>QTDMSRKAFVFPKESDTSYVSLKAPLTKPLKAFTVCLHFYTELSSTRGYSIFSYATKRQDNEILIFWSKDIGYSFTVGGSEILFEVPEVTVAPVHICTSWESASGIVEFWVDGKPRVRKSLKKGYTVGAEASIILGQEQDSFGGNFEGSQSLVG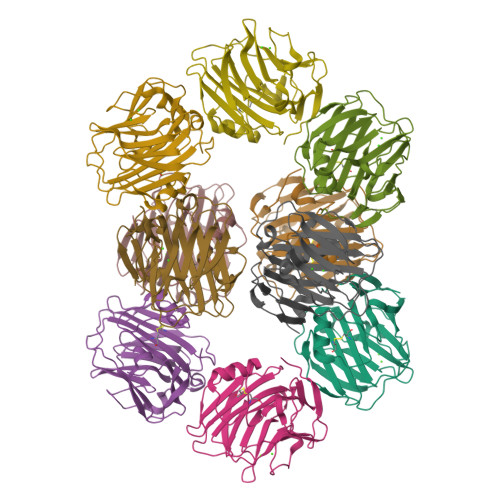DIGNVNMWDFVLSPDEINTIYLGGPFSPNVLNWRALKYEVQGEVFTKPQLWP[10x]> MSEIGTGFPFDPHYVEVLGERMHYVDVGPRDGTPVLFLHGNPTSSYLWRNIIPHVAPSHRCIAPDLIGMGKSDKPDLDYFFDDHVRYLDAFIEALGLEEVVLVIHDWGSALGFHWAKRNPERVKGIACMEFIRPIPTWDEWPEFARELFQAFRTADVGRELIIDQNAFIEQVLPKFVVRPLTEVEMDHYREPFLKPVDREPLWRFPNELPIAGEPANIVALVEAYMNWLHQSPVPKLLFWGTPGVLIPPAEAARLAESLPNCKTVDIGP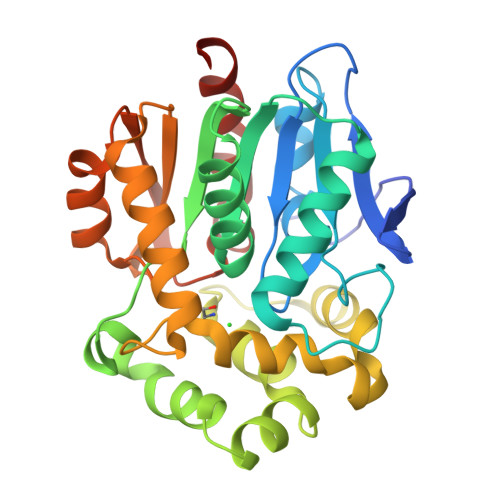GLHYLQEDNPDLIGSEIARWLPALHHHHHH>[2x]MGASDDLTIEILTDDADYDLQRFDCGEEALNLFLTTHLVRQHRNKILRAYILCRNTPERQVLGYYTLCGSCFERAAL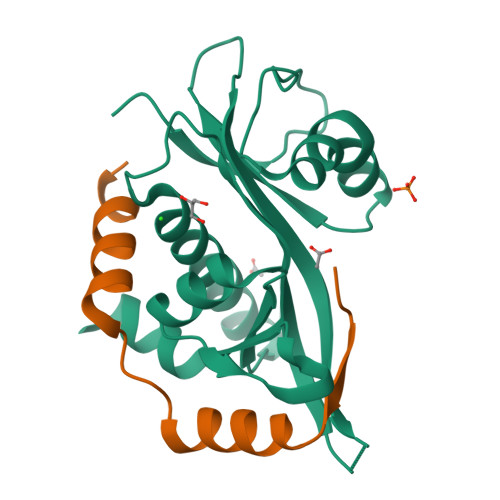PSKSKQKKIPYKNIPSVTLGRLAIDRSLQGQGWGATLVAHAMNVVWSASLAVGIHGLFVEALNEKAHTFFKSLGFIPLVGENENALFFPTKSIELLFTQSD;>[2x]MAAEVIEQHRRVILNEESWTRVMDALSNPPSPGEKLKRAAKRLQGM> GQANHPTAAVVTEKQQMLEQHLQDVRKRVQDLEQKMKVVENLQDDFDFNYKTLKSQGDMQDLNGNNQSVTRQKMQ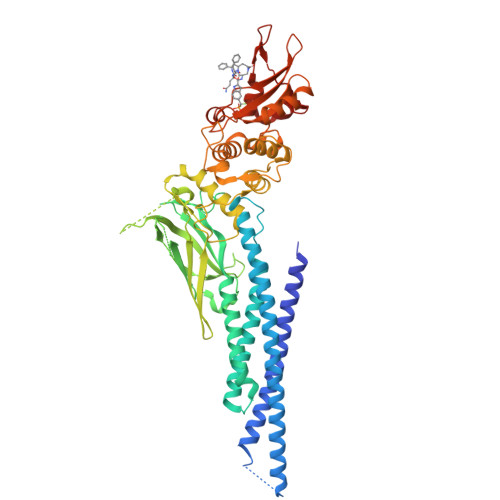QLEQMLTALDQMRRSIVSELAGLLSAMEYVQKTLTDEELADWKRRQQIACIGGPPNICLDRLENWITSLAESQLQTRQQIKKLEELQQKVSYKGDPIVQHRPMLEERIVELFRNLMKSAFVVERQPCMPMHPDRPLVIKTGVQFTTKVRLLVKFPELNYQLKIKVCIDKDSGDVAALRGSRKFNILGTNTKVMNMEESNNGSLSAEFKHLTLREQRCGNGGRANCDASLIVTEELHLITFETEVYHQGLKIDLETHSLPVVVISNICQMPNAWASILWYNMLTNNPKNVNFFTKPPIGTWDQVAEVLSWQFSSTTKRGLSIEQLTTLAEKLLGPGVNYSGCQITWAKFCKENMAGKGFSFWVWLDNIIDLVKKYILALWNEGYIMGFISKERERAILSTKPPGTFLLRFSESSKEGGVTFTWVEKDISGKTQIQSVEPYTKQQLNNMSFAEIIMGYKIMDATNILVSPLVYLYPDIPKEEAFGKYCR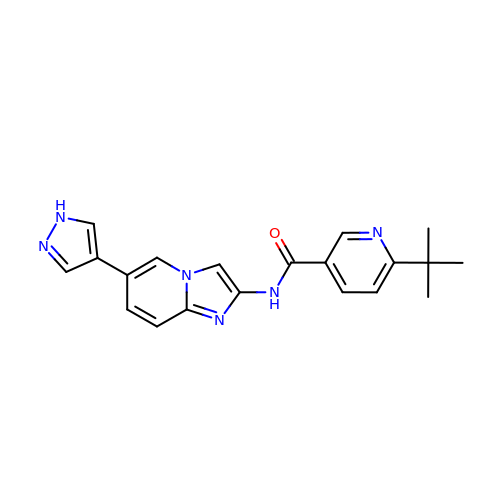6-~{tert}-butyl-~{N}-[6-(1~{H}-pyrazol-4-yl)-1~{H}-imidazo[1,2-a]pyridin-2-yl]pyridine-3-carboxamide | C20 H20 N6 O | BNBGXFKXNXXHEZ-UHFFFAOYSA-N Protocadherin-19 (PCDH19) is a member of the non-clustered δ2-protocadherin subfamily that is located on the X-chromosome. Mutations in PCDH19 cause an X-linked, female-limited form of infant-onset epilepsy (PCDH19 female epilepsy, PCDH19-FE; OMIM 300088) that is associated with intellectual disability, as well as compulsive or aggressive behavior and autistic features. However, PCDH19 along with the rest of the non-classical cadherins lack these critical tryptophan residues and must mediate adhesion by an alternative mechanism. Here we present crystals structures of the highly homologous zebrafish Protocadherin-19 (Pcdh19) encompassing repeats EC1-4 and EC3-4.

One of the Pcdh19 EC3-4 molecules was used to solve the Pcdh19 EC1-4 structure (3.59 Å), which contains two molecules in the asymmetric unit, each starting from Val one to Asp 422 (RMSD of 1.4 Å). The EC1 repeat has a disulfide bond at the E-F loop, typical of clustered protocadherins, as well as one of two α-helices (at the B-C loop) also found in structures of clustered protocadherins. The three linker regions of Pcdh19 (EC1-2, EC2-3, EC3-4) have canonical cadherin calcium-binding sites. There are 51 PCDH19-FE missense mutations (out of 70) that can be mapped to 43 locations in the Pcdh19 EC1-4 structure. Pcdh19 EC1-4 crystals were grown from the putative dimer SEC peak elution, and two plausible adhesive interfaces are observed in our Pcdh19 EC1-4 structure. The first one, which we will refer to as Pcdh19-I1, arises from contacts between the two Pcdh19 EC1-4 molecules in the asymmetric unit, and involves a fully-overlapped antiparallel dimer in which EC1 from one molecule interacts with EC4 from the other (EC1:EC4), EC2 with EC3 (EC2:EC3), EC3 with EC2 (EC3:EC2), and EC4 with EC1 (EC4:EC1). Analysis of the Pcdh19-I1 antiparallel interface with the Protein Interfaces, Surfaces and Assemblies (PISA) server and with the NOXclass classifier revealed a large interface (~1650 Å2), that is unlikely to be a crystal packing artifact (89.21% biological, 81% obligate). The Pcdh19-I1 interface involves extended and mostly symmetric, in-register contacts between repeats EC2:EC3 that account for ~58% of the interfacial area, as well as smaller, separate EC1:EC4 contacts (~350 Å2 × 2) that are slightly off-register. Taken together, our crystallographic structural analyses and binding assays including PCDH19-FE mutations strongly support a model in which fully overlapped EC1-4 domains (Pcdh19-I1 interface) form the functional adhesive unit of Pcdh19. The antiparallel Pcdh19-I1 dimer interface validated above reveals a homophilic 'forearm handshake' binding mechanism for PCDH19, involving overlap of 4 ECs from each protomer wrapping around each other.

>MVFNLKYTVEEELRAGTKIANVTADAKVAGFALGNRQPYLRVISNSEPRWVNLSPAGLLITKQKIDRDAVCRQTPKCFISLEVMSNSMEICVIKIEIIDVNDNAPRFPTNHIDIEISENAAPGTRFPLEGASDPDSGSNGIQTYTITPNDIFGLEIKTRGDGSKIAELVVEKTLDRETQSRYTFELTAEDGGDPPKSGTVQLNIKVIDSNDNNPVFDEPVYTVNVLENSPINTLVIDLNATDPDEGTNGEVVYSFINFVSNLTKQMFKIDPKTGVITVNGVLDHEELHIHEIDVQAKDLGPNSIPAHCKVIVNVIDINDNAPEIKLLSENSEMVEVSENAPLGYVIALVRVSDNDSGANGKVQCRLQGNVPFRLNEFESFSTLLVDGRLDREQRDMYNLTILAEDSGYPPLRSSKSFAVKVTDLEHHHHHH[2x]When building atomic models into weak and/or low-resolution density, a common strategy is to restrain their conformation to that of a higher resolution model of the same or similar sequence. When doing so, it is important to avoid over-restraining to the reference model in the face of disagreement with the experimental data. Here, two new such potentials are described: a Cartesian distance restraint derived from a recent generalization of common loss functions and a periodic torsion restraint based on a renormalization of the von Mises distribution. Further, their implementation as user-adjustable/switchable restraints in ISOLDE is described and their use in some real-world examples is demonstrated.

We performed a three-dimensional grid search over reasonable values of springConstant, angleRange and alpha using the following protocol, with three technical replicates for each combination of parameters. The resulting coordinates were then refined in phenix.refine (six refinement rounds of reciprocal-space xyz and individual B-factor refinement, using the starting coordinates as a reference model). To define ‘incorrect’ residues, we compared each model with our manually rebuilt and refined exemplar using a backbone and side-chain torsion scoring system that we defined for the assessment of CASP13 model predictions (Croll et al., 2019; for backbones the average of unit chord lengths arising from Δφ, Δψ and Δω; for side chains a weighted average of Δχ1 and Δχ2 chord lengths adjusted for the degree to which the side chain is buried). In each case an ‘incorrect’ residue was defined as one with a score higher than 0.15 (approximately equivalent to an average deviation of ±45° from the exemplar). Since R free is only poorly correlated with model quality in low-resolution models, optimization on this parameter alone is inadvisable. Instead, we considered four individual read-outs of model quality: R free (fit to data), MolProbity score (general stereochemical quality) and match to the exemplar at the backbone and side-chain level. There is no apparent correlation between R free and the latter three measures for this data set. The point marked in red indicates the values we chose as default (springConstant = 250, angleRange = 60, alpha = 0.3), representing the lowest (i.e. most conservative) value for each parameter yielding close to optimal results for each read-out.

> QFHVKSGLQIKKNAIIDDYKVTSQVLGLGINGKVLQIFNKRTQEKFALKMLQDCPKARREVELHWRASQCPHIVRIVDVYENLYAGRKCLLIVMECLDGGELFSRIQDRGDQAFTEREASEIMKSIGEAIQYLHSINIAHRDVKPENLLYTSKRPNAILKLTDFGFAKETTSHNSLTTPCYTPYYVAPEVLGPEKYDKSCDMWSLGVIMYILLCGYPPFYSNHGLAISPGMKTRIRMGQYEFPNPEWSEVSEEVKMLIRNLLKTEPTQRMTITEFMNHPWIMQSTKVPQTPLHTSRVLKEDKERWEDVKEEMTSALATMRVDYEQIK>[2x]MTILIIAGILGFIMAFSIGANDVANSMATAVGARAITVRQAALIAMFLEFLGAVMFGSHVSQTIVKGIVEVEKVQPVELMYGALSALIAASFWILIATNWGYPVSTTHSIVGGMM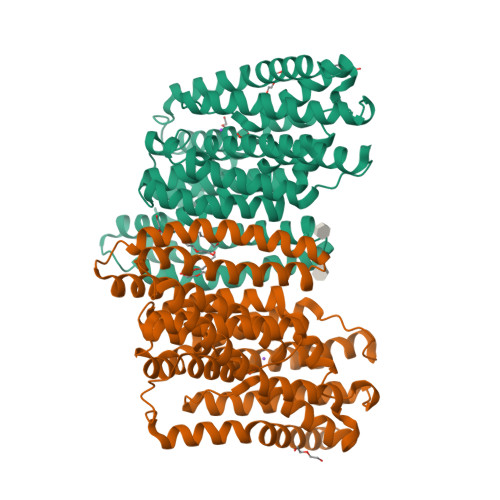GFGLVAVGINGVNWKTFLFIVLSWVVSPVLGGLISFVMFKLISLSVFHTKNPKKSSTVAIPFFISLAIFTMISLFVKKTLKQPLSESFLLGIAFSLVTFFVVHFAVRKLINEKKDVYDAVENVFKRAQILTSCYVSFSHGANDVANAAGPVAAVMIVASTGVVPKTVEIPFLALLLGGIGISLGVFFLGQKVMETVGEKITTLTNSRGFTVDFSTATTVLLASSLGLPISTTHVVVGAVTGVGFARGLEMVNVGVLKNIVISWLLIVPTVAATSAAVYWVLKLILKF> TTSGALFPSLVPGSRGASNKYLVEFRAGKMSLKGTTVTPDKRKGLVYIQQTDDSLIHFCWKDRTSGNVEDDLI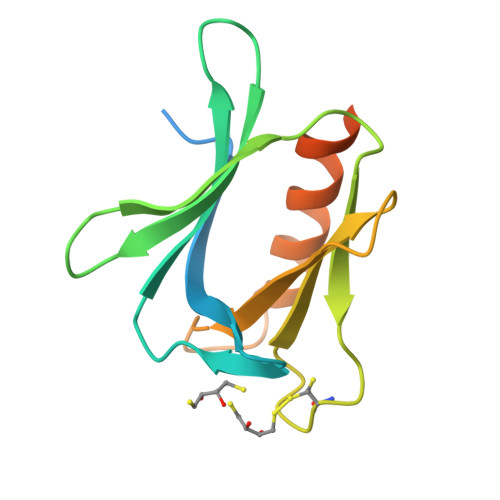IFPDDCEFKRVPQCPSGRVYVLKFKAGSKRLFFWMQEPKTDQDEEHCRKVNEYLNNPPMPGALGASGSSGHELSAL>MKYFLDSAILEEIRYAYENWAIDGVTTNPRHIMNSGKPFLTVLDEFASEFKGVENFPISVEINPHLDNAKDMVEEGTKIAKLSSNFVIKIPCTEPGLIAAKEFEKQGISTNVTLVFSPSQALQPARIGAKFVSPFVGWKENSGDDTTQYIQDIVNIYKNYNYNTEIIVAALRNGKQIVDAAKAGAHI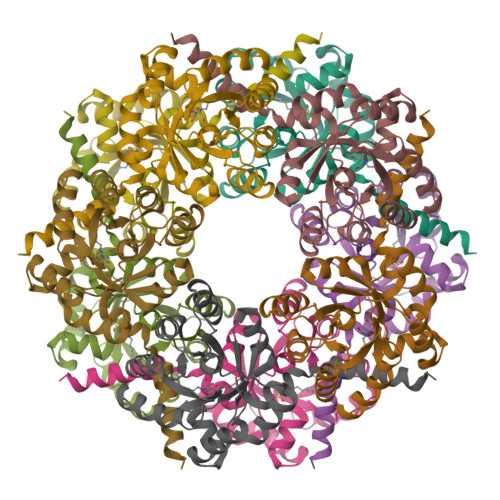VTCGFDVYKESFQHAFTDYGLNKFRNAWDNTVTEAPVLK[10x]> MASARGYVNIKTFEQKLDGNKKIEGKEVSVAFPLYSDVHKISGAHYQTFPSEKAAYSTVYE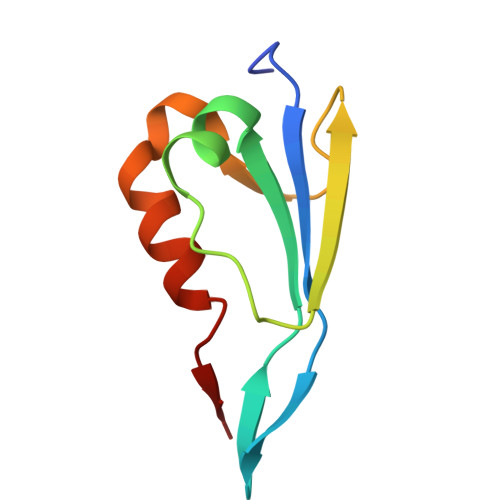ENQRTEWIAANEDLWKVTG>MSQPRGGRGGGRGGGVGRKTPSSLTGPPDESATPSERATPASKADSDPKDDSSSNGDKKDMDLFPAPKPPSAGASIRDTANKVLGLAMKSEWTPIEAELKKLEKYVANVGEDGNHIPLAGVHDMNTGMTPLMYATKDNKTAIMDRMIELGADVGARNNDNYNVLHIAAMYSREDVVKLLLTKRGVDPFSTGGSRSQTAVHLVSSRQTGTATNILRALLAAAGKDIRLKADGRGKIPLLLAVESGNQSMCRELLAAQTAEQLKATTANGDTALHLAARRRDVDMVRILVDYGTNVDTQNGEGQTPLHIAAAEGDEALLKYFYGVRASASIADNQDRTPMHLAAENGHAHVIEILADKFKASIFERTKDGSTLMHIASLNGHAECATMLFKKGVYLHMPNKDGARSIHTAAAYGHTGIINTLLQKGEKVDVTTNDNYTALHIAVESAKPAVVETLLGFGADVHVRGGKLRETPLHIAARVKDGDRCALMLLKSGASPNLTTDDCLTPVHVAARHGNLATLMQLLEDEGDPLYKSNTGETPLHMACRACHPDIVRHLIETVKEKHGPDKATTYINSVNEDGATALHYTCQITKEEVKIPESDKQIVRMLLENGADVTLQTKTALETAFHYCAVAGNNDVLMEMISHMNPTDIQKAMNRQSSVGWTPLLIACHRGHMELVNNLLANHARVDVFDTEGRSALHLAAERGYLHVCDALLTNKAFINSKSRVGRTALHLAAMNGFTHLVKFLIKDHNAVIDILTLRKQTPLHLAAASGQMEVCQLLLELGANIDATDDLGQKPIHVAAQNNYSEVAKLFLQQHPSLVNATSKDGNTCAHIAAMQGSVKVIEELMKFDRSGVISARNKLTDATPLQLAAEGGHADVVKALVRAGASCTEENKAGFTAVHLAAQNGHGQVLDVLKSTNSLRINSKKLGLTPLHVAAYYGQADTVRELLTSVPATVKSETPTGQSLFGDLGTESGMTPLHLAAFSGNENVVRLLLNSAGVQVDAATIENGYNPLHLACFGGHMSV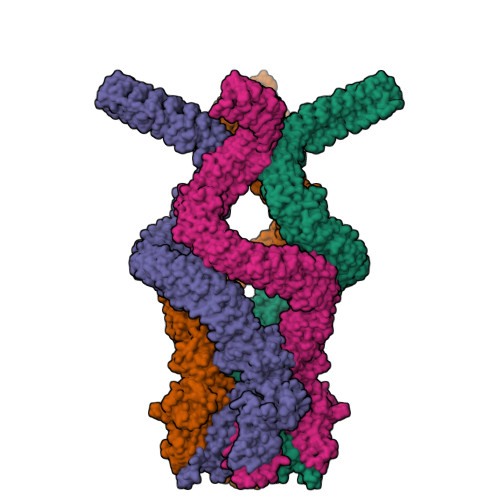VGLLLSRSAELLQSQDRNGRTGLHIAAMHGHIQMVEILLGQGAEINATDRNGWTPLHCAAKAGHLEVVKLLCEAGASPKSETNYGCAAIWFAASEGHNEVLRYLMNKEHDTYGLMEDKRFVYNLMVVSKNHNNKPIQEFVLVSPAPVDTAAKLSNIYIVLSTKEKERAKDLVAAGKQCEAMATELLALAAGSDSAGKILQATDKRNVEFLDVLIENEQKEVIAHTVVQRYLQELWHGSLTWASWKILLLLVAFIVCPPVWIGFTFPMGHKFNKVPIIKFMSYLTSHIYLMIHLSIVGITPIYPVLRLSLVPYWYEVGLLIWLSGLLLFELTNPSDKSGLGSIKVLVLLLGMAGVGVHVSAFLFVSKEYWPTLVYCRNQCFALAFLLACVQILDFLSFHHLFGPWAIIIGDLLKDLARFLAVLAIFVFGFSMHIVALNQSFANFSPEDLRSFEKKNRNRGYFSDVRMHPINSFELLFFAVFGQTTTEQTQVDKIKNVATPTQPYWVEYLFKIVFGIYMLVSVVVLIQLLIAMMSDTYQRIQAQSDIEWKFGLSKLIRNMHRTTTAPSPLNLVTTWFMWIVEKVKARMKKKKRPSLVQMMGIRQASPRTKAGAKWLSKIKKDSVALSQVHLSPLGSQASFSQANQNRIENVADWEAIAKKYRALVGDEEGGSLKDSDAESGSQEGSGGQQPPAQVGRRAIKATLADTTK[4x]>[4x]GPLGSMADAAPQLGKRKRELDVEEAHAASTEEKEAGVGNGTCAPVRLPFSGFRLQKVLRESARDKIIFLHGKVNEASGDGDGEDAVVILEKTPFQVEQVAQLLTGSPELQLQFSNDIYSTYHLFPPRQLNDVKTTVVYPATEKHLQKYLRQDLRLIRETGDDYRNITLPHLESQSLSIQWVYNILDKKAEADRIVFENPDPSDGFVLIPDLKWNQQQLDDLYLIAICHRRGIRS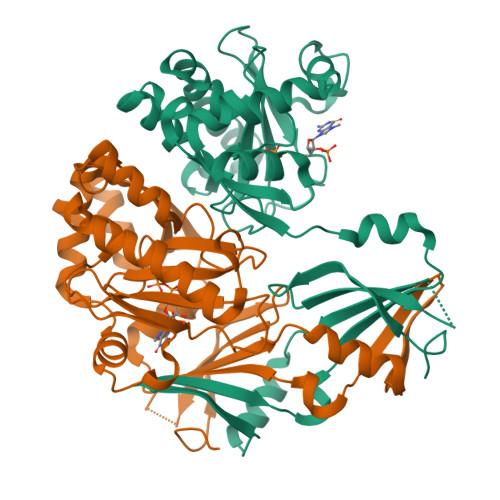LRDLTPEHLPLLRNILHQGQEAILQRYRMKGDHLRVYLHYLPSYYHLHVHFTALGFEAPGSGVERAHLLAEVIENLECDPRHYQQRTLTFALRADDPLLKLLQEAQQS> KVVAGTEFPISLGSKISTVVKRPKQKKRSKKAKEDEEEILVIEGIEFDRDVAVKFDVYVNDVDDLPSGPDKTEFAGSFVSVPHS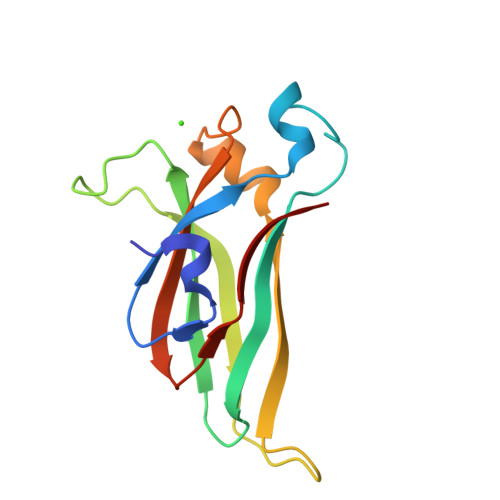HKHKKKMNTILRLGLTDLLEEIEAEDDDSVVVTLVPKFGAVKIGGIKIEFAS Cypoviruses, members of the family Reoviridae, subfamily Spinareovirus, possess a single capsid layer with turrets and are commonly embedded in crystalline occlusion bodies called polyhedra, which are formed in the cell cytoplasm and mainly composed of a single virus-encoded protein, polyhedrin. To ensure the delivery of virus particles to the target intestinal cells, allowing the transmission of packages of infectious virus between hosts by oral-faecal routes, polyhedra are disrupted only when they are exposed to the very alkaline pH environment found in insect midguts. The fold of all the polyhedrins is highly similar – a β-barrel core sitting on a base domain, surrounded by a common array of five helices (H1–H5). The strongest intermolecular interactions define a trimer composed of a cluster of three β-barrels sandwiched by helices top and bottom.

As expected from the 83% amino acid sequence identity, CPV18 looks very similar to CPV1. The exception is the polyhedrin of CPV18, which has >80% sequence identity with that of CPV1, consistent with their relatively recent divergence. In CPV18 purine binding is almost identical to CPV1 in that GTP hydrogen bonds with V2c and V1 while ATP is supported by two V4 regions from different polypeptide chains. The ATP and GTP bases stack with each other and with the phenol ring of Y172. There are two substitutions in the binding pocket, K154H and R155V. Residue 155 interacts via the main chain nitrogen, and is thus sequence independent, whilst at residue 154 both the lysine and histidine side chain NH groups hydrogen bond with ATP phosphates. Despite a strong overall similarity with CPV1 there is no pyridine bound in CPV18. Many of the key residues that bind the CTP in CPV1 (H76, N77, D78, S79, Y80, D81, D96 and R98) are substituted, including H76N and S79P, which interact with the phosphates and R98T which stacks with the base. Clearly these changes are sufficient to disrupt CTP binding. Although the two molecules are very similar (rmsd of 247 structurally equivalent Cαs 0.23 Å) they behave dramatically differently in alkali buffers, CPV18 being far more sensitive to dissolution.

> MADVAGTSNRDFRGREQRLYNSEQYNYNNSLNGEVSLWVYAYYSDGSVLVRNCNSQYKVGISECFKSLKEVRVGQNNDPYDEQEVNNGVYYPNGGEPTKFHSNAKPRAIQIIFSPSVNVHTIKMAKGNSVSIPKDYLQRSHPWEATGVKYRKIHVDGEIVGYSHYFELPHEYNSISLSVSGVHKNPSSYNVAAPHNIMDVFQSCDLALKFSNRYWCELELINHYISAYAYPYLDINNHKYGVPLNGRQ>NPPMFSQDVFSVTLREDVPPGFSVLQVTATDQDEGVNAEITYAFHNVDEQVERIFNLDKRTGEITTKDNLDFETAKSYTLNVEAKDPGDLASHCSIQVKILDENDCVPEVIVTSVFTPLPEDSPLGTVIALIKTRDRDSGENGDVYCHVLGNEGFVLKSSSKNYYKLVTDRTLDREAIPEYNVTIVAADRGKPPLSSNVIITLHISDVNDNAPVFHQASYLVHVAENNPPGTSIAQVSASDPDLGSNGLISYSIIASDLEPRALSSFVSVNQDSGVVFAQRAFDHEQLRSFQLTLQARDHGSPTLSANVSMRVLVGDRNDNAPRVLYPTLEPDGSALFDMVPRAAEPGYLVTKVVAVDADSGHNAWLSYHVLQASDPGLFSLGLRTGEVRTARALGDRDSARQRLLVAVRDGGQPPLSATATLHLIFADSLQEHHHHHHHH[3x]

By contrast, in vertebrates the clustered protocadherins (Pcdhs) provide analogous cell-surface diversity, but in this case generated through stochastic alternative promoter choice. Biophysical measurements with domain-deleted proteins showed that Pcdhs also interact in cis, through a membrane-proximal dimer interface involving extracellular cadherin domain 6 (EC6) and potentially EC5. The specificity-determining cell-cell recognition interface of Pcdhs involves domains EC1–4, as shown experimentally through mutagenesis analysis and suggested by mutation correlation analysis.

From these experiments we obtained crystals of γA4EC3–6 and γB2EC3–6, which diffracted to sufficient resolution for crystal structure determination. The resolution of the final refined structures was 3.0/4.3/2.85 Å for γA4EC3–6 and 2.3 Å for γB2EC3–6. The two structures are similar overall (RMSD of 3.02 Å over 405 Cα’s), although γA4EC3–6 shows a more pronounced EC4–EC5 bend angle (32.6° for γA4 vs. 18.6° for γB2). These are the first Pcdh structures containing EC6, which displays the classic beta sandwich fold, but with a large insertion between the A and A’ strands. However the γB2EC3–6 crystal structure also did not reveal any interactions with clear biological relevance. Since γB2EC3–6 forms a weak cis dimer in solution (80.1 μM), this was unexpected. The monomeric arrangement in the crystal is likely an artifact of crystallization, perhaps due to the low pH of the crystallization condition (pH 6.5). Furthermore, O-mannosylation is observed at EC6 G-strand residues 624, 626, and 628 (γB2 numbering) of both the γB2 and γA4 structures—on the opposite molecular face to the mutations that disrupt cell surface delivery.> MASLTVKAYLLGKEDAAREIRRFSFSFSPEPEAEAEAAAGPGP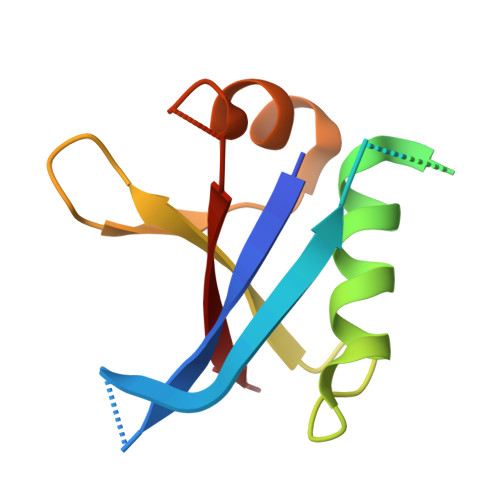CERLLSRVAALFPALRPGGFQAHYRAERGDLVAFSSDEELTMAMSYVKDDIFRIYIKEK>MDYKDDDDKMSRRFTVTSLPPAGPARSPDPESRRHSVADPRHLPGEDVKGDGNPKESSPFINSTDTEKGKEYDGKNMALFEEEMDTSPMVSSLLSGLANYTNLPQGSREHEEAENNEGGKKKPVQAPRMGTFMGVYLPCLQNIFGVILFLRLTWVVGIAGIMESFCMVFICCSCTMLTAISMSAIATNGVVPAGGSYYMISRSLGPEFGGAVGLCFYLGTTFAGAMYILGTIEILLAYLFPAMAIFKAEDASGEAAAMLNNMRVYGTCVLTCMATVVFVGVKYVNKFALVFLGCVILSILAIYAGVIKSAFDPPNFPICLLGNRTLSRHGFDVCAKLAWEGNETVTTRLWGLFCSSRFLNATCDEYFTRNNVTEIQGIPGAASGLIKENLWSSYLTKGVIVERSGMTSVGLADGTPIDMDHPYVFSDMTSYFTLLVGIYFPSVTGIMAGSNRSGDLRDAQKSIPTGTILAIATTSAVYISSVVLFGACIEGVVLRDKFGEAVNGNLVVGTLAWPSPWVIVIGSFFSTCGAGLQSLTGAPRLLQAISRDGIVPFLQVFGHGKANGEPTWALLLTACICEIGILIASLDEVAPILSMFFLMCYMFVNLACAVQTLLRTPNWRPRFRYYHWTLSFLGMSLCLALMFICSWYYALVAMLIAGLIYKYIEYRGAEKEWGDGIRGLSLSAARYALLRLEEGPPHTKNWRPQLLVLVRVDQDQNVVHPQLLSLTSQLKAGKGLTIVGSV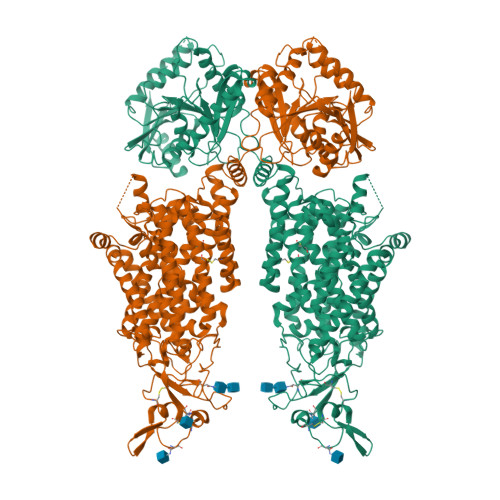LEGTFLENHPQAQRAEESIRRLMEAEKVKGFCQVVISSNLRDGVSHLIQSGGLGGLQHNTVLVGWPRNWRQKEDHQTWRNFIELVRETTAGHLALLVTKNVSMFPGNPERFSEGSIDVWWIVHDGGMLMLLPFLLRHHKVWRKCKMRIFTVAQMDDNSIQMKKDLTTFLYHLRITAEVEVVEMHESDISAYTYEKTLVMEQRSQILKQMHLTKNEREREIQSITDESRGSIRRKNPANTRLRLNVPEETAGDSEEKPEEEVQLIHDQSAPSCPSSSPSPGEEPEGEGETDPEKVHLTWTKDKSVAEKNKGPSPVSSEGIKDFFSMKPEWENLNQSNVRRMHTAVRLNEVIVKKSRDAKLVLLNMPGPPRNRNGDENYMEFLEVLTEHLDRVMLVRGGGREVITIYSWSHPQFEK[2x]> MELRHIRYFLAVAEERHFTRAAARLGIGQPPLSQQIKDLERELGALLFRRVSYGAELTEAGIAFLDVVKEIPVMAERATQAAQRAVRGELGVLRVGFTASSAFNSVVPTAIRAFRRAYPDVRLQLEEDNTTRLADGLNEGSLDVAFLRPGFAGSERFHLRMLSEEPMMIVMAENHPAASYEEISLSAFRDETFLLFPREIGLTLYDSVIESCRTAGFEPTIGQLAPQIASVINLVAAEMGVSIVPASMSQVKVIGVVYRHIADQTPTAKLALAYRRGDTSPVLRNFVLTVFP

The bacterial protein ItcR is unique in its ability to bind to itaconate. Structurally, ItcR is a transcriptional regulator protein with an N-terminal DNA-binding helix-turn-helix motif and a C-terminal itaconate-binding domain (IBD)24. Multiangle light scattering (MALS) analysis showed that IBD appears as homodimer in solution. Here, we report the development of a highly responsive, genetically encoded itaconate fluorescent biosensor, referred to as BioITA (biosensor for itaconate).

The IBD was expressed in Escherichia coli and purified by affinity chromatography and gel filtration. Furthermore, the crystal structure of IBD without or with itaconate binding was determined by multiple-wavelength anomalous diffraction and refined at a resolution of 3.25 and 1.48 Å, respectively. In line with the result of MALS, the IBD proteins form a homodimer in both of the apo and itaconate bound states. Notably, alignment between the structures of IBD in the apo and itaconate bound states demonstrated that monomer in each dimer exhibited translocation of over 7 and 10 Å in the N- and C-termini, respectively.> MTGNPDPNANPNVDPNANPNANPNANPNANPNANPNAEPSDKHIKEYLNKIQNSLSTEWSPCSVTCGNGIQVRIKPGSANKPKDELDYANDIEKKICKME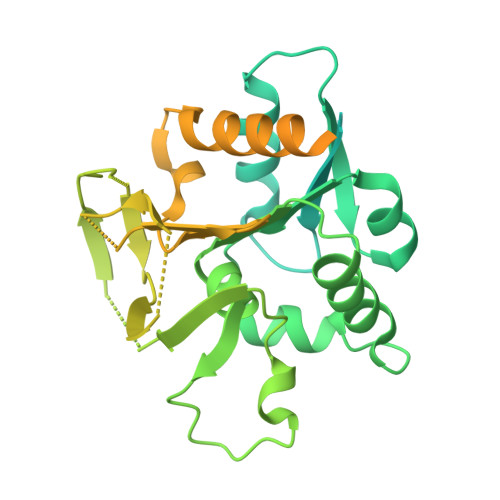KCSSVFNVVNSGGSGTEITIGVLSLQGDFEPHINHFIKLQIPSLNIIQVRNVHDLGLCDGLVIPGGESTTVRRCCAYEQDTLYNALVHFIHVLKKPIWGTCAGCILLSKNVENIKLYSNFGNKFSFGGLDITICRNFYGSQQDSFICSLNIISDSSAFKKDLTAACIRAPYIREILSDEVKVLATFSHESYGPNIIAAVEQNNCLGTVFNPELLPHTAFQQYFYEKVKNYKYSTGNPDPNANPNVDPNANPNANPNANPNANPNANPNAEPSDKHIKEYLNKIQNSLSTEWSPCSVTCGNGIQVRIKPGSANKPKDELDYANDIEKKICKMEKCSSVFNVVNSGGSLEHHHHHH>MIISEFDRNNPVLKDQLSDLLRLTWPEEYGDSSAEEVEEMMNPERIAVAAVDQDELVGFIGAIPQYGITGWELHPLVVESSRRKNQIGTRLVNYLEKEVASRGGITIYLGTDDLDHGTTLSQTDLYEHTFDKVASIQNLREHPYE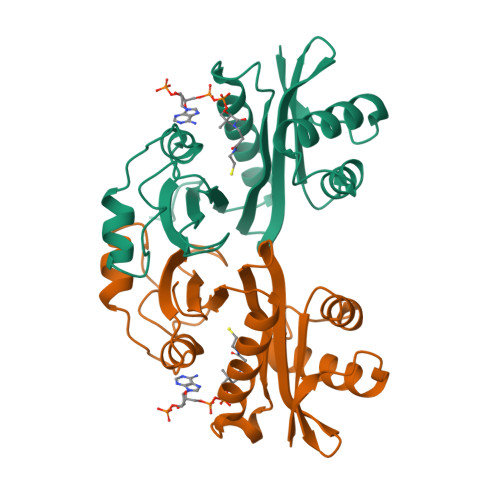FYEKLGYKIVGVLPNANGWDKPDIWMAKTIIPRPD[4x]> MNSTNSGPPDSGSATGVVPTPDEIASLLQVEHLLDQRWPETRIDPSLTRISALMDLLGSPQRSYPSIHIAGTNGKTSVARMVDALVTALHRRTGRTTSPHLQSPVERISIDGKPISPAQYVATYREIEPLVALIDQQSQASAGKGGPAMSKFEVLTAMAFAAFADAPVDVAVVEVGMGGRWDATNVINAPVAVITPISIDHVDYLGADIAGIAGEKAGIITRAPDGSPDTVAVIGRQVPKVMEVLLAESVRADASVAREDSEFAVLRRQIAVGGQVLQLQGLGGVYSDIYLPLHGEHQAHNAVLALAS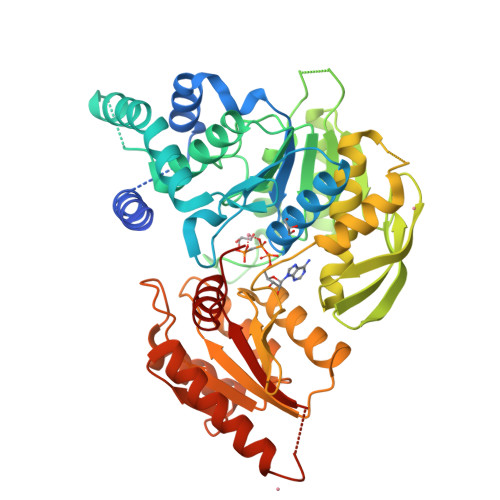VEAFFGAGAQRQLDGDAVRAGFAAVTSPGRLERMRSAPTVFIDAAHNPAGASALAQTLAHEFDFRFLVGVLSVLGDKDVDGILAALEPVFDSVVVTHNGSPRALDVEALALAAGERFGPDRVRTAENLRDAIDVATSLVDDAAADPDVAGDAFSRTGIVITGSVVTAGAARTLFGRDPQ>[2x]CGCAAATTTGCG

The rational design of small molecules that target specific DNA sequences is a promising strategy to modulate gene expression. This report focuses on a diamidinobenzimidazole compound, whose selective binding to the minor groove of AT DNA sequences holds broad significance in the molecular recognition of AT-rich human promoter sequences. The specialized method of X-ray crystallography was utilized to investigate how the sequence-dependent recognition properties in general, A-tract, and alternating AT sequences affect the binding of diamidinobenzimidazole in the DNA minor groove. A strong and direct hydrogen bond between the N-H of the benzimidazole and an H-bond acceptor atom in the minor groove is essential for DNA recognition in all sequences described. In addition, the diamidine compound specifically utilizes an interfacial water molecule for its DNA binding.

Like most AT-tract minor grooves, AAATTT DNA has a high propeller twist in the AT region, which in many cases correlates to a narrower minor groove.>[5x]GLFEGDKFVGSFESAAMGTFVIDMRSYETLVNSTSLDRIKSYANSFNKYKY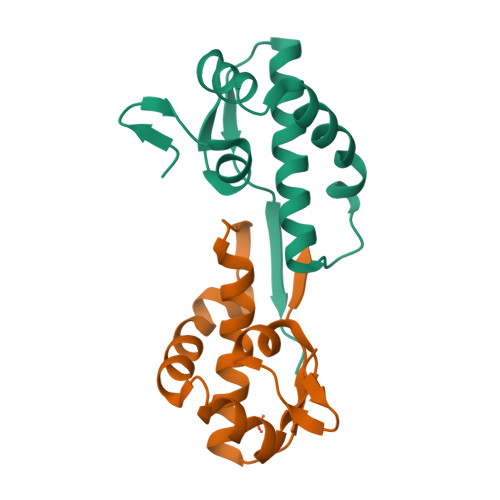YTGSMGEADYRMACYAHLGKALMDYSVSRNDKLYTPPTVSVNSTL> MAHHHHHHMTDATAGKIPHVLVIMDGVGHREAIEDNAFLAAKTPNLTAMKAKHPNSLISGSGEDVGLPDGQMGNSEVGHMNLGAGRVLYQDFTRITKDIRTGAFFEHEVLVDAVEKAKAAGGAVHIMGLLSEGGVHSHEDHIVAMCELALKRGAKVYLHAFLDGRDTPPRSAQPSLEKLDALFAQYEGKGRIATMIGRYFAMDRDNRWDRVEQAYRLLTEGEAVRTATTAVEGLELAYAANENDEFVKATRIGEIAKVQDGDSVVFMNFRADRAREITRAFVEKDFAGFERKVVPNLSKFVMLTRYQASIDAPVAYMPEELKNSLGEYLSSLGKTQLRIAETEKYAHVTFFFSGGREDEYPGEKRILIPSPNVATYDLKPEMSAYEVTDELVKAINSGEYDLLVVNYANGDMVGHTGVFDAAVKAVEAVDTCLGRVYEAVMAKKGHMLITADHGNVEQMQDYES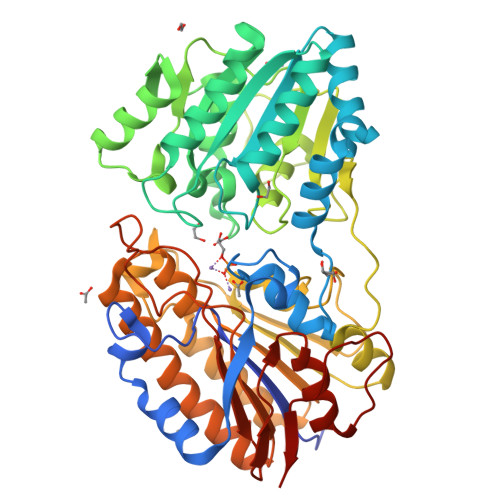GQVHTQHTTELVPFIYVGPTQATIAEGGVLADVAPTILNLMQIPVPAEMQGRNLITLSA>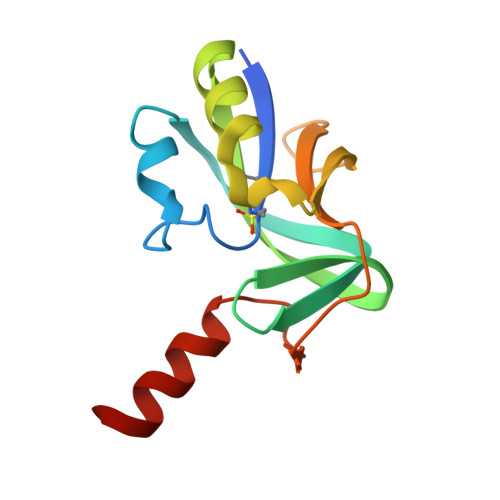 MSYKEKSVRIAVYGTLRKGKPLHWYLKGAKFLGEDWIEGYQLYFEYLPYAVKGKGKLKVEVYEVDKETFERINEIEIGTGYRLVEVSTKFGKAFLWEWGSKPRGKRIKSGDFDEIRLEHHHHHH>GPGHMDPDTFSYNFNNRPILSRRNTVWLCYEVERLDNGTWVKMDQHRGQVYSELKYHPEMRFLSLVSKWKLHRDQEYEVTWYISWSPCTKCARDMATFLQENTHVTLTIFVARLYYFWDPDYQEALRSLAQAGATIKIMNYDEFQHCWSKFVYSQGAPFQPWDGLDEYSQALSGMLGEILRHSMDPPTFTFNFNNEPWVRGRHETYLCYEVERMHNDTWVKLNQRRGFLANQAPHKHGFLEGRHAELCFLDVIPFWKLDLDQDYRVTCFTSWSPCFSCAQEMAKFISKNKHVSLCIKTARIYDDQGRAQEGLRTLAEAGAKISIMTYSEFKHCWDTFVDHQGAPFQPWDGLDEHSQDLSGRLRAILQNQEN[2x];>MGSSHHHHHHSQDPMENRWQVMIVWQVDRMRINTWKRLVKHHMYISRKAKDWFYRHHYESTNPKISSEVHIPLGDAKLVITTYWGLHTGERDWHLGQGVSIEWRKKRYSTQVDPDLADQLIHLHYFDEASEGSQIKPPLPSVRKLTEDRWNK[4x];>MPRVVPDQRSKFENEEFFRKLSRECEIKYTGFRDRPHEERQARFQNACRDGRSEIAFVATGTNLSLQFFPASWQGEQRQTPSREYVDLEREAGKVYLKAPMILNGVCVIWKGWIDLQRLDGMGCLEFDEERAQQEDALAQQAFEEARRRTREFEDR[4x]

HIV-1 hijacks a host ubiquitin ligase complex using a viral infectivity factor, Vif, to degrade the antiviral factor, APOBEC3G (A3G). A3G is a human, single-stranded DNA (ssDNA) deaminase that catalyzes fatal mutations in genomes of viruses such as HIV-1 [Reviewed in 6–9]. Here we show reconstitution of the A3G-Vif complex and subsequent A3G ubiquitination in vitro and report the cryo-EM structure of the A3G-Vif complex at 2.8 Å resolution using solubility-enhanced variants of A3G and Vif. In summary, our high-resolution cryo-EM structure of sA3G-VC-RNA20 revealed that Vif binds sA3G through interactions with ssRNA.

The refined C2-symmetrized map reaches 2.8 Å resolution and allows us to build an atomic model unambiguously. In the asymmetric unit of this sA3G-VC-RNA20 structure, a single sA3G assembles with two VCs, named VCred and VCblue. On the other hand, the sA3G-VCred-RNA20 interface involves neither mutations nor heterodimer interactions; therefore, it most likely reveals biologically relevant interactions. The protein-protein interface of sA3G-Vifred is biologically pivotal for complex formation because it includes A3G amino acid D128, which has been identified as a determinant of species-specific A3G-Vif interaction. Our cryo-EM structure shows sA3G side chains D128 and D130 proximal to the side chain of R15 located in Vifred helix α1, suggesting that their rotamers form bifurcated hydrogen bonds. The preceding sA3G residue, W127, makes contact with Vifred H43, forming a π-π interaction between the aromatic rings. The dinucleotide rG6rA7 is located at the sA3G-Vifred interface. The well-resolved nucleotide, rA7, is buried deeper and is accommodated in the pocket of sA3G NTD formed by NTD loops α1/β1 and β4/α4. In addition, the 2′-hydroxyl group of rG6 ribose can form bifurcated hydrogen bonds with side chains H42 and H43 of Vifred. We tested deaminase activity on ssRNA by sA3G, but no rC deaminase reaction was observed using in vitro deamination assay, even though base rC9 points toward the pseudo-catalytic pocket of sA3G NTD.>[2x]DEWPEPIVRVQSLAESNLSSLPDRYIK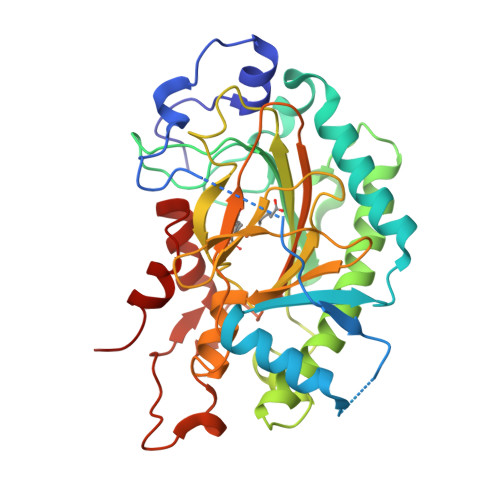PASLRPTTTEDAPTATNIPIIDLEGLFSEEGLSDDVIMARISEACRGWGFFQVVNHGVKPELMDAARENWREFFHMPVNAKETYSNSPRTYEGYGSRLGVEKGASLDWSDYYFLHLLPHHLKDFNKWPSFPPTIREVIDEYGEELVKLSGRIMRVLSTNLGLKEDKFQEAFGGENIGACLRVNYYPKCPRPELALGLSPHSDPGGMTILLPDDQVFGLQVRKDDTWITVKPHPHAFIVNIGDQIQILSNSTYKSVEHRVIVNSDKERVSLAFFYNPKSDIPIQPLQELVSTHNPPLYPPMTFDQYRLFIRTQGPQGKSHVESHISP>[4x]LGKRSLRKMWRPGEKKEPQGVVYEDVPDDTEDFKESLKVVFEGSAYGLQNFNKQKKLKRCDDMDTFFLHYAAAEGQIELMEKITRDSSLEVLHEMDDYGNTPLHCAVEKNQIESVKFLLSRGANPNLRNFNMMAPLHIAVQGMNNEVMKVLLEHRTIDVNLEGENGNTAVIIACTTNNSEALQILLKKGAKPCKSNKWGCFPIHQAAFSGSKECMEIILRFGEEHGYSRQLHINFMNNGKATPLHLAVQNGDLEMIKMCLDNGAQIDPVEKGRCTAIHFAATQGATEIVKLMISSYSGSVDIVNTTDGCHETMLHRASLFDHHELADYLISVGADINKIDSEGRSPLILATASASWNIVNLLLSKGAQVDIKDNFGRNFLHLTVQQPYGLKNLRPEFMQMQQIKELVMDEDNDGCTPLHYACRQGGPGSVNNLLGFNVSIHSKSKDKKSPLHFAASYGRINTCQRLLQDISDTRLLNEGDLHGMTPLHLAAKNGHDKVVQLLLKKGALFLSDHNGWTALHHASMGGYTQTMKVILDTNLKCTDRLDEDGNTALHFAAREGHAKAVALLLSHNADIVLNKQQASFLHLALHNKRKEVVLTIIRSKRWDECLK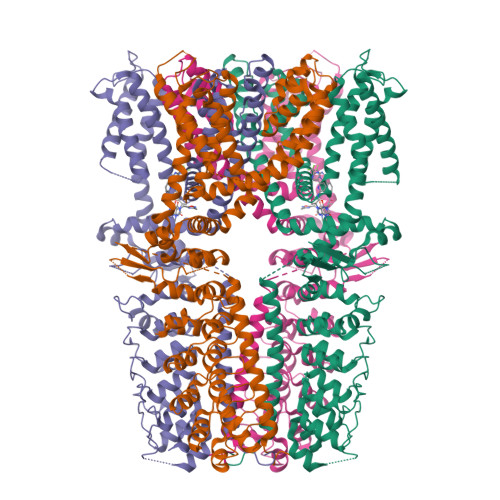IFSHNSPGNKCPITEMIEYLPECMKVLLDFCMLHSTEDKSCRDYYIEYNFKYLQCPLEFTKKTPTQDVIYEPLTALNAMVQNNRIELLNHPVCKEYLLMKWLAYGFRAHMMNLGSYCLGLIPMTILVVNIKPGMAFNSTGIINETSDHSEILDTTNSYLIKTCMILVFLSSIFGYCKEAGQIFQQKRNYFMDISNVLEWIIYTTGIIFVLPLFVEIPAHLQWQCGAIAVYFYWMNFLLYLQRFENCGIFIVMLEVILKTLLRSTVVFIFLLLAFGLSFYILLNLQDPFSSPLLSIIQTFSMMLGDINYRESFLEPYLRNELAHPVLSFAQLVSFTIFVPIVLMNLLIGLAVGDIAEVQKHASLKRIAMQVELHTSLEKKLPLWFLRKVDQKSTIVYPNKPRSGGMLFHIFCFLFCTGEIRQEIPNADKSLEMEILKQKYRLKDLTFLLEKQHELIKLIIQKMEIISETEDDDSHCSFQDRFKKEQMEQRNSRWNTVLRAVKAKTHHLEP> MELQQNFTDNNSIKYTAILILIAFAFSVLARLYWVAWASEFYEFFFNDQLMITTNDG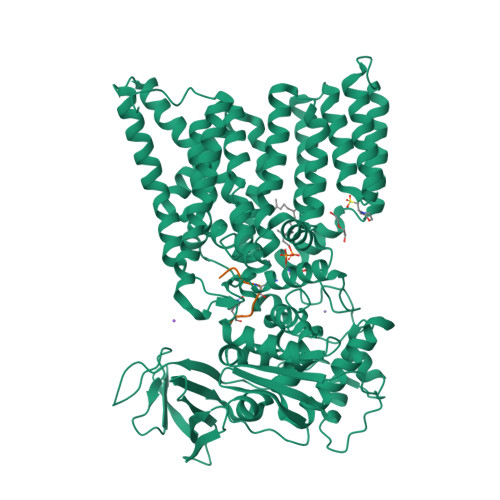YAFAEGARDMIAGFHQPNDLSYFGSSLSTLTYWLYSILPFSFESIILYMSTFFASLIVVPIILIAREYKLTTYGFIAALLGSIANSYYNRTMSGYYDTDMLVLVLPMLILLTFIRLTINKDIFTLLLSPVFIMIYLWWYPSSYSLNFAMIGLFGLYTLVFHRKEKIFYLTIALMIIALSMLAWQYKLALIVLLFAIFAFKEEKINFYMIWALIFISILILHLSGGLDPVLYQLKFYVFKASDVQNLKDAAFMYFNVNETIMEVNTIDPEVFMQRISSSVLVFILSFIGFILLLKDHKSMLLALPMLALGFMALRAGLRFTIYAVPVMALGFGYFLYAFFNFLEKKQIKLSLRNKNILLILIAFFSISPALMHIYYYKSSTVFTSYEASILNDLKNKAQREDYVVAWWDYGYPIRYYSDVKTLIDGGKHLGKDNFFSSFVLSKEQIPAANMARLSVEYTEKSFKENYPDVLKAMVKDYQKTSAKDFLESLNDPNFKIDTPKTRDVYIYMPYRMLRIMPVVAQFANTNPDNGEQEKSLFFSQANPLDQDKKQGSITLDNGVEISNDYRSLKIEGNSIPLKAFVDIESITNGKFYYNEIDSKAQIYLLYLREYKSYVILDESLYNSSYIQMFLLNQYDQDLFEQITNDTRAKIYRLKREFHHHHHHHHHH;> GDQAATFG>[2x]MVKRTSHKQASCPVARPLDVIGDGWSMLIVRDAFEGLTRF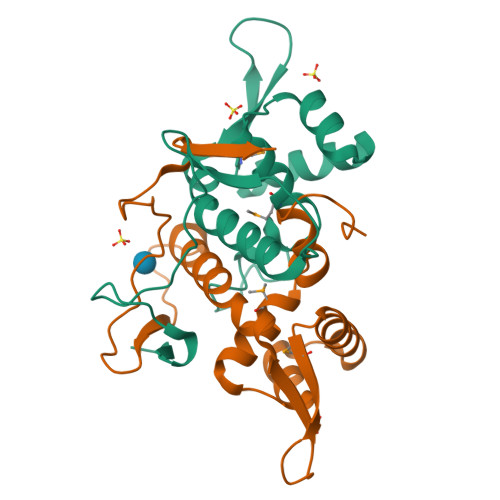GEFQKSLGLAKNILAARLRNLVEHGVMVAVPAESGSHQEYRLTDKGRALFPLLVAIRQWGEDYFFAPDESHVRLVERDSGQPVPRLQVRAGDGSPLAAEDTRVSRD>MASEKHFKYVILGGGVAAGYAAREFAKQGVKPGELAIISKEAVAPYERPALSKGYLFPQNAARLPGFHVCVGSGGERQLPEWYSEKGIELILSTEIVKADLSTKTLTSAAGATFTYEILIIATGSSVIKLTDFGTQGADSNNILYLREIDDADKLVAAIQAKKGGKAVVVGGGYIGLELSAALKINDFDVTMVFPEPWCMPRLFTADIAAFYEAYYTNKGVKVLKGTLAVGFDANANGDVTAVKLKDGKVLEADIVVVGVGGRPLTTLFKGQVAEEKGGIKTDAFFETSVPGVYAIGDVATFPLKMYNELRRVE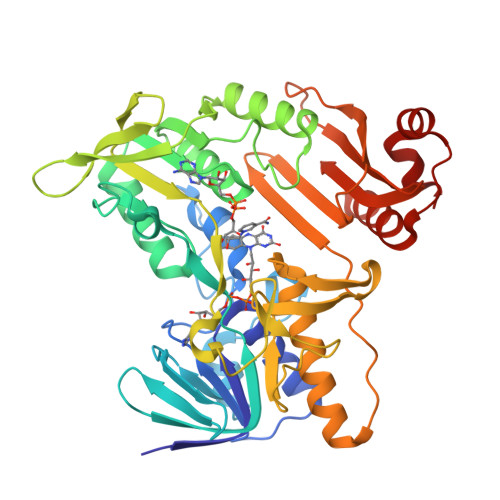HVDHSRKSAEQAVKAIKGKESGESVPEYDYLPYFYSRSFDLGWQFYGDNVGETILFGDSDPTSSKPKFGSYWIKDGKVFGAFLEGGSPDENNAIAKVAKTQPPVASIEELKKEGLQFASKI[2x]2-ACETAMIDO-5-(4-PHENYLPHENYL)BENZOIC ACID | C21 H17 N O3 | 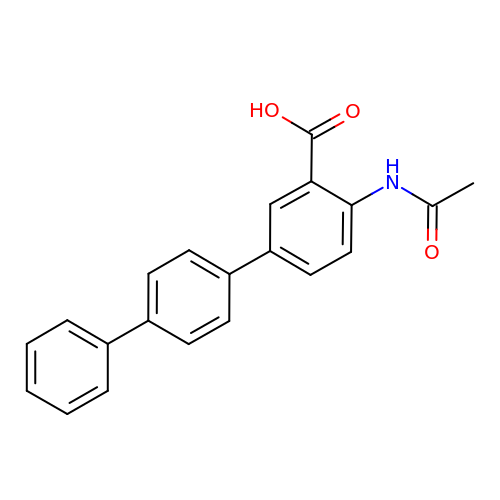XXPKIBVYLUEVCV-UHFFFAOYSA-N>[4x]SMMNLLRRSGKRRRSESGSDSFSGSGGDSSASPQFLSGSVLSPPPGLGRCLKAAAAGECKPTVPDYERDKLLLANW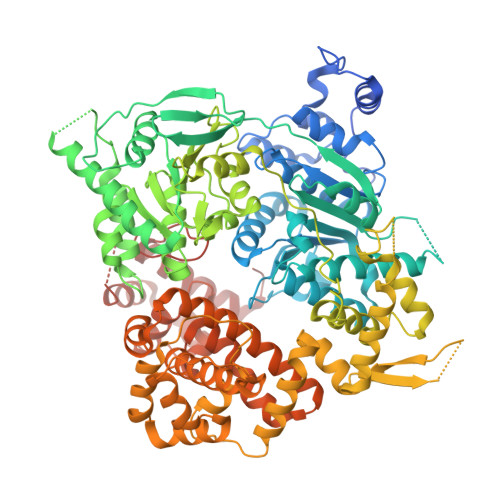GLPKAVLEKYHSFGVKKMFEWQAECLLLGQVLEGKNLVYSAPTSAGKTLVAELLILKRVLEMRKKALFILPFVSVAKEKKYYLQSLFQEVGIKVDGYMGSTSPSRHFSSLDIAVCTIERANGLINRLIEENKMDLLGMVVVDELHMLGDSHRGYLLELLLTKICYITRKSASCQADLASSLSNAVQIVGMSATLPNLELVASWLNAELYHTDFRPVPLLESVKVGNSIYDSSMKLVREFEPMLQVKGDEDHVVSLCYETICDNHSVLLFCPSKKWCEKLADIIAREFYNLHHQAEGLVKPSECPPVILEQKELLEVMDQLRRLPSGLDSVLQKTVPWGVAFHHAGLTFEERDIIEGAFRQGLIRVLAATSTLSSGVNLPARRVIIRTPIFGGRPLDILTYKQMVGRAGRKGVDTVGESILICKNSEKSKGIALLQGSLKPVRSCLQRREGEEVTGSMIRAILEIIVGGVASTSQDMHTYAACTFLAASMKEGKQGIQRNQESVQLGAIEACVMWLLENEFIQSTEASDGTEGKVYHPTHLGSATLSSSLSPADTLDIFADLQRAMKGFVLENDLHILYLVTPMFEDWTTIDWYRFFCLWEKLPTSMKRVAELVGVEEGFLARCVKGKVVARTERQHRQMAIHKRFFTSLVLLDLISEVPLREINQKYGCNRGQIQSLQQSAAVYAGMITVFSNRLGWHNMELLLSQFQKRLTFGIQRELCDLVRVSLLNAQRARVLYASGFHTVADLARANIVEVEVILKNAVPFKSARKAVDEEEEAVEERRNMRTIWVTGRKGLTEREAAALIVEEARMILQQDLVEM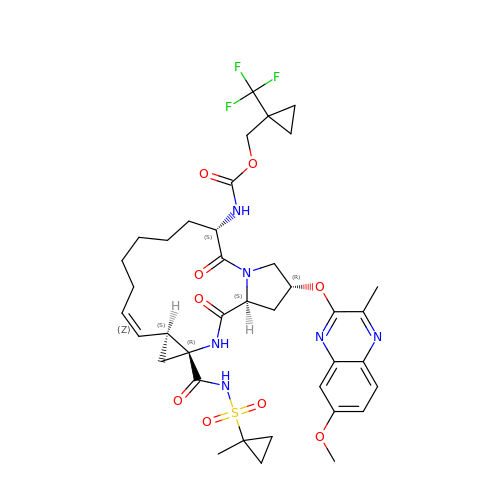[1-(trifluoromethyl)cyclopropyl]methyl {(2R,4S,6S,12Z,13aS,14aR,16aS)-2-[(7-methoxy-3-methylquinoxalin-2-yl)oxy]-14a-[(1-methylcyclopropane-1-sulfonyl)carbamoyl]-5,16-dioxo-1,2,3,5,6,7,8,9,10,11,13a,14,14a,15,16,16a-hexadecahydrocyclopropa[e]pyrrolo[1,2-a][1,4]diazacyclopentadecin-6-yl}carbamate | C38 H47 F3 N6 O9 S | OIRPWGZAWBASNA-RVJOZYONSA-N>[4x]HGFVSGAVVDGKYYTGYLVNQYPYMSSPPESIGWSETATDLGFVDGSGYSSGDIICHKSAKNGAISAEIKAGGKVEFQWTEWPESHHGPVITYMANCNGDCASVDKTSLEF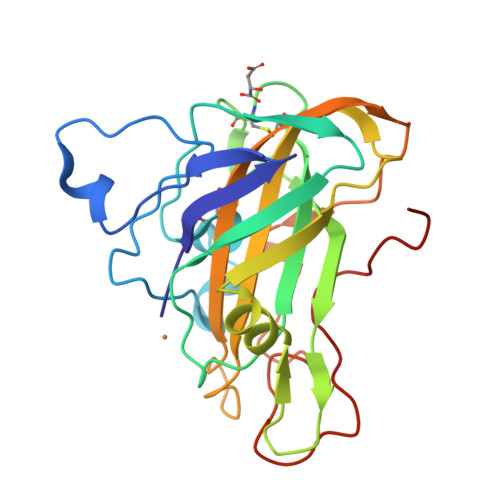FKIDESGLISDSNVPGTWASDNLIANNNSWTVTVPSSIAAGNYVMRHEIIALHSAGNQNGAQNYPQCINLKVTGGGSDKPAGTLGTALYKNTDAGILVNIYQSLSSYDIPGPALYSGHHHHHH>[2x]MVKVDLESKRYGEKLKEVFLMLDNNVVECIKEITESSRNGKLVFFVGAGVSTLSDYPQWWRLVDKYHEELYGSPKKGNYSSDEYLRIPQIFYNVKGEMAFDGILKDFFQVDKPTNPIHDKILAMNPAHVITTNYDNLIDTACWKRGKYFSVISAEEDVANATSSRYLLKVHGD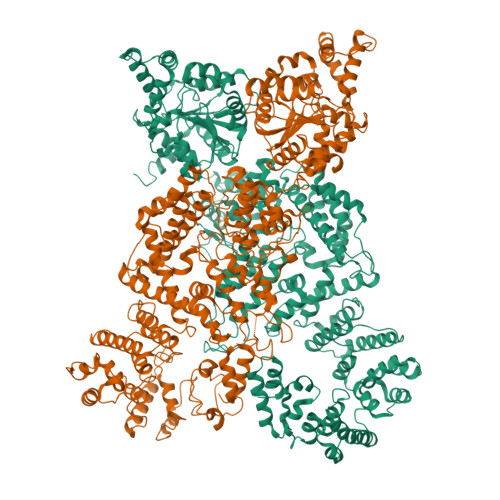FRKGFKGENVVLKEDDYLNYDQNYPLISNLMKTIIATHTIVFIGYGLGDYNINMLLNWVRKLQKDSFHKPFFIRTDPSPIENETLIYYENKGLRIIDAASLIDSNEYDYLERYSAVMDLLIESQENKFITKDDEVIDYIYGKISPLFALQYIRKIDLKHVFEYDYHFEVNGTVVRHKNKGFGYMERFFELKESCDERSKLSKKQYERFNALFNFFEKNGVICMAKDAGTLNTSIEINSLAYHGKYDVMKKFIEEQSVSIEDDYKKAFFLACLGRWEESYDLYSNIILNSIDESNGCVYYLSQINRYRIYQSITQAVTQFNGLGLLTFGRHYKPFTDEFLARIEREMTNFNIDDLFNGMPFEFQKKYKILEFLSDNQFLYDDTVKLFELTNKVRSEMSEGSYSFGMSSDIVVLLRLYDNLRFLYENCLWSVSFHEFHQYIRNSMSLLIEKAEYERTRDIDELGFSFFGKKSGFFMEYYDFVNISRHFKIDDIKNLERSCSIDKIRFGEQEKIEEYLVGIAEEITKQFSANGMNVVFYTQFISEAKAALYFAKYVKLSEEGLGKIVKALLFYFPERDLDIGKRYVWLERLTKCNELPKSIISIIDDFLVLQAEKHIDQNYSEVSSNGLYSRDYGALIKHFEKNFISKRLSEITLCLTQDKQKQIDFLFKLLPLLSTNAKSHLLSFKSVENINDLMNGIRIGLIDEFTPEHEELIIEYLETRKVNYIVEKEKGIQTFSSNDYMSTFGIWYFLEEINNSKMEEFIGMDDQYDFFVDPENFDYKKFIPSWLKNYNDKLLGKIAGNKHMKHHVIEVLKERVKNSNDKRYLEILMNYFI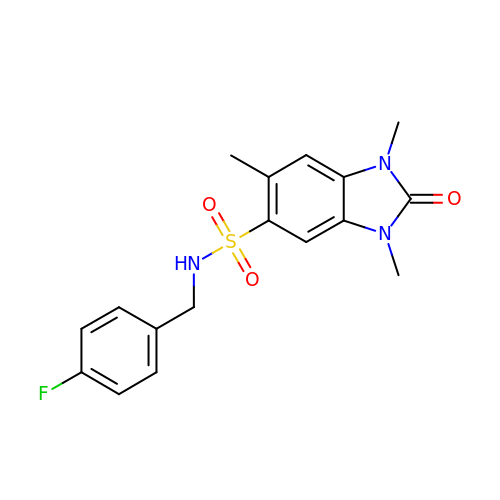~{N}-[(4-fluorophenyl)methyl]-1,3,6-trimethyl-2-oxidanylidene-benzimidazole-5-sulfonamide | C17 H18 F N3 O3 S | HJRSXSGULYKETP-UHFFFAOYSA-N> GSGPPGPPGPPGPPGARGQAGVMGF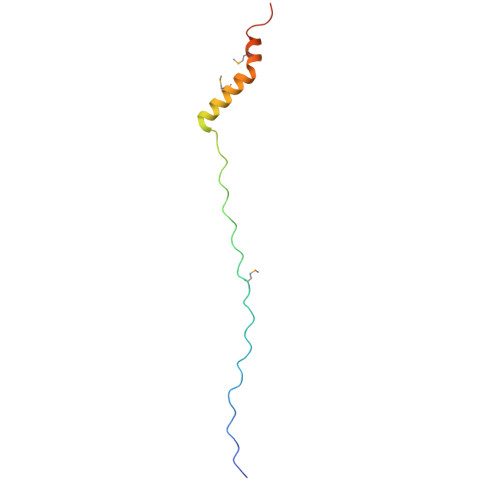PGPPGPPGPPGRAPTDQHIKQVCMRVIQEHFAEMAASLKRPDSGAT>MFEGFERRLVDVGDVTINCVVGGSGPALLLLHGFPQNLHMWARVAPLLANEYTVVCADLRGYGGSSKPVGAPDHANYSFRAMASDQRELMRTLGFERFHLVGHARGGRTGHRMALDHPDSVLSLAVLDIIPTYVMFEEVDRFVARAYWHWYFLQQPAPYPEKVIGADPDTFYEGCLFGWGATGADGFDP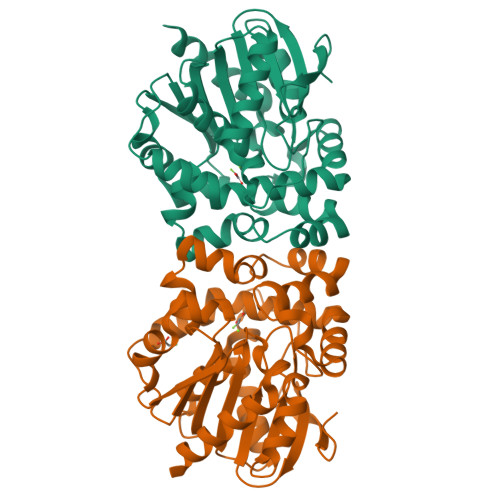EQLEEYRKQWRDPAAIHGSCCDYRAGGTIDFELDHGDLGRQVQCPALVFSGSAGLMHSLFEMQVVWAPRLANMRFASLPGGHFFVDRFPDDTARILREFLSDARSGIHQTERRES[2x]>[2x]SAEQVEKLRNKINNAAVLVFAKSFCPYCKKVMERFNNLKIPFGYLDLDLKKNGSDYQKMLQEITGRTTVPQVFFRGEFIGGCDDVMAIDDDTIVKKANEMKYDYDMVIIGGGSGGLALAKESAKSGAKVALLDFVVPTPMGTTWGLGGTCVNVGCIPKKLMHQAALLNHYMEDAKSFGWDVDKGPHDWVKMVEGIQDHIHALNFGYRSSMMNANVKYLNALGEIVDPHTIKTTNKQGIVKNITTNTII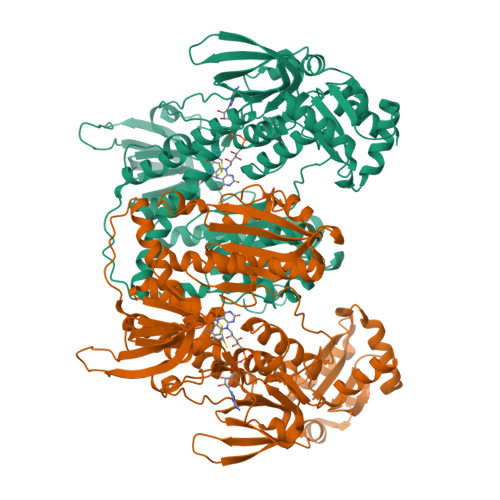VATGERPRYPPIPGAKEYGITSDDLFTLDHNPGKTLCVGASYVSLECAGFLSSIGCDVTVMVRSIFLRGFDQQMAGLISDYIAKYGVKFVRPCVPTSVRCLEEYDPESGKLAIYEVEGKHEDGTPFKDTFNTVLFAVGRDPCTTNIGLQNVDVKTTNGRVVVDDEERTNVPNIYAIGDVSNAGYQLTPLAIQAGKNLARRLYTADDCRTDYTNVPTTVFTPLEYGCIGLSEENAISKFGEDNIEVFHSYFQPLEWTVPHRPDNTCYAKLIINKQDDNRVVGFHVFGPNAGEVTQGYAVAMHLGARKEDFDRTIGIHPTCSETFTTLRVTKSSGASA> MHHHHHHGGESKKRQWALEDFEIGRPLGKGKFGNVYLAREKQSKFILALKVLFKAQLEKAGVEH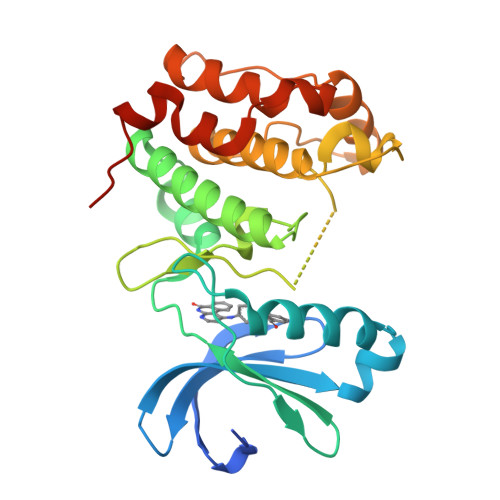QLRREVEIQSHLRHPNILRLYGYFHDATRVYLILEYAPLGTVYRELQKLSKFDEQRTATYITELANALSYCHSKRVIHRDIKPENLLLGSAGELKIADFGWSVHAPSSRRTTLCGTLDYLPPEMIEGRMHDEKVDLWSLGVLCYEFLVGKPPFEANTYQETYKRISRVEFTFPDFVTEGARDLISRLLKHNPSQRPMLREVLEHPWITANSSKPSNCQNK> VIEKVQHIQLLQKNVRAQLVDMKRLEVDIDIKIRSCRGSC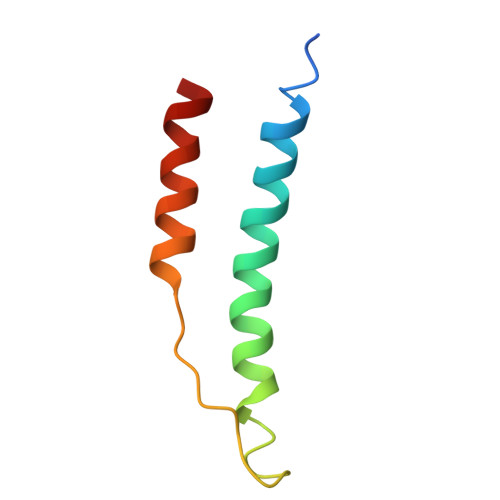SRALAREVDLKDYEDQQKQLEQVIAK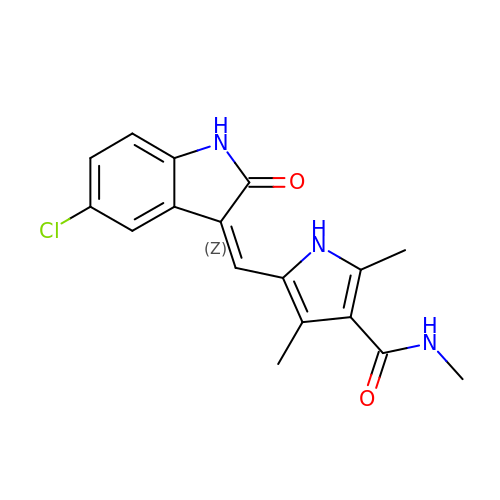5-[(Z)-(5-CHLORO-2-OXO-1,2-DIHYDRO-3H-INDOL-3-YLIDENE)METHYL]-N-(DIETHYLAMINO)ETHYL]-2,4-DIMETHYL-1H-PYRROLE-3-CARBOXAMIDE | C17 H16 Cl N3 O2 | FIRPCWHHIWFKCD-GHXNOFRVSA-N>GGGTGGGTGGGTTGGGTTAGCGTTA[4x];>[4x]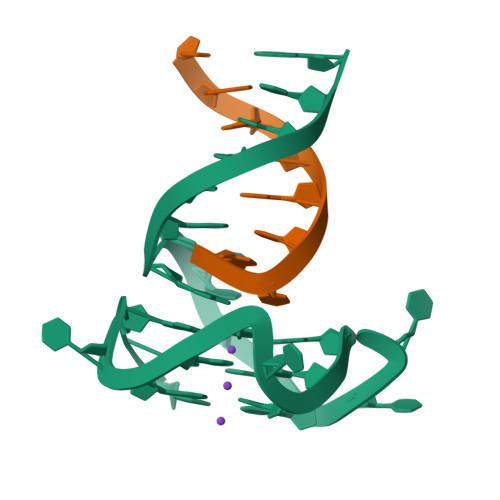TAACGCTA> MRGSHHHHHHGSAVSAKIEIYTWSTCPFCMRALALLKRKGVEFQEYCIDGDNEAREAMAARANGKRSLPQIFIDDQHIGGCDDIYALDGAGKLDRLLHS

In the case of the glutaredoxin that is the focus of this study, glutaredoxin A from the cyanobacterium Synechocystis sp. PCC 6803 serves as the preferred electron donor for the 2-electron reduction of arsenate to arsenite, catalyzed by arsenate reductase. As part of the thioredoxin superfamily, glutaredoxin A shares the characteristic thioredoxin fold. The structure of the wild-type protein is comprised of the major protein secondary structure elements: four α-helical segments, and four mixed parallel: anti-parallel β-strands that form a single β-pleated sheet. Our random mutagenesis approach has yielded four new crystal structures of glutaredoxin A, one for each of the following variants: R27L, A75I, A79S, and P84R.

The P84R mutation is interesting from a structural perspective. Firstly, Pro84 occurs at the beginning of an α-helix that is bent by almost 90° relative to a neighboring α-helix in the structure. The only impetus for this dramatic bend is the maintenance of a protected hydrophobic core. A proline is present at this locus in other glutaredoxin molecules, but not all. As proline does not provide a free backbone amide hydrogen to form an H-bond to the i + 4 backbone carbonyl, it rarely occurs within a helix. In the wild-type glutaredoxin structure, there is only one i, i + 4 backbone H-bond interaction to stabilize α-helix 4. While mutation of Pro84 to arginine does not restore the complete backbone H-bond pattern typical of α-helices, it does appear to alleviate strain on the peptide backbone so an additional i, i + 4 backbone H-bond interaction can form between the backbone carbonyl of Asp83 and the backbone amine of Ser88. The R27L crystal structure lacks two neighbors; the A75I and A79S mutant have no net differences, while the P84R mutant adds three possible interactions.> MRGSHHHHHHGSQLPISPIETVPVKLKPGMDGPKVKQWPLTEEKIKALVEICTEMEKEGKISKIGPENPYNTPVFAIKKKDGTKWRKLVDFRELNKKTQDFWEVQLGIPHPAGLKKKKSVTVLDVGDAYFSVPLDEDFRKYTAFTIPSINNETPGIRYQYNVLPQGWKGSPAIFQSSMTKILEPFRKQNPDIVIYQYMDDLYVGSDLEIGQHRTKIEELRQHLLRWGLTTPDKKHQKEPPFLWMGYELHPDKWTVQPIVLPEKDSWTVNDIQKLVGKLNWASQIYPGIKVRQLCKLLRGTKALTEVIPLTEEAELELAENREILKEPVHGVYYDPSKDLIAEIQKQGQGQWTYQIYQEPFKNLKTGKYARMRGAHTNDVKQLTEAVQKITTESIVIWGKTPKFKLPIQKETWETWWTEYWQATWVPEWEFVNTPPLVKLWYQLEKEPIVGA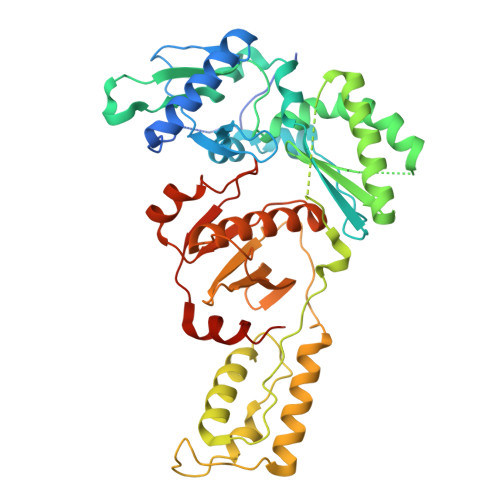ETF> MPRTPHLLAIQSHVVFGHAGNAAAVFPMQRIGINVWPLNTVQFSNHTQYGRWTGQVLPPEQIPALVDGIAGIGELGNCDAVLSGYLGSAAQGRAILDVVARIKQ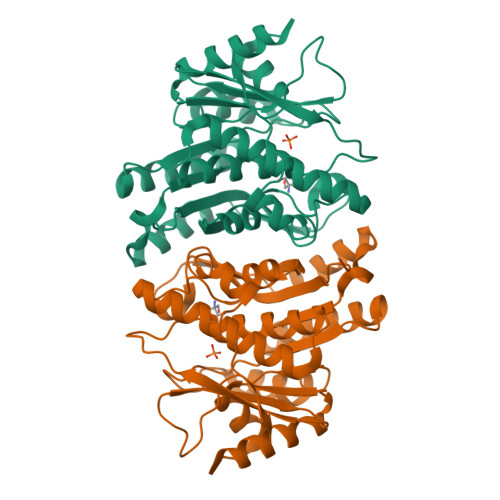ANPRALYLCDPVMGHPEKGCIVAPEVSDFLLEEAAAVADYLCPNQLELDSFCDRQPNSLADCVEMARSLLARGPRAILVKHLNYPGKAGDTFEMLLVAADQAWHLQRPLLAFPRQPVGVGDLASGLFLSRLLLGDDLRNAFEFTGAAVHEVLLETQACGSYELELVRAQDRIAHPRVRFDAVRL> SYYAVAVVKKGTDFMIKDLRGKTSCHTGLGRSAGWNIPIGTLIHREDIEWE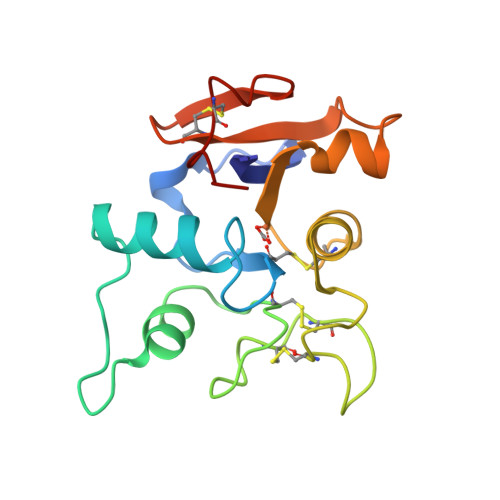GIESGSVEQAVAKFFSASCVPGATIEQKLCRQCKGDAKTKCLRNAPYSGYSGAFQCLKDGKGDVAFVKHTTVQENAPEEKDEYELLCLDGSRQPVDSYKTCNWARVAA> QVQSVEVMRDSYGVPHVFADSHYGLYYGYGYAVAQDRLFQMDMARRSFVGTTAAVLGPGEQDAYVKYDMQVRQNFTPASIQRQIAALSKDERDIFRGYADGYNAYLEQVRRRPELLPKEYVDFDFQPEPLTDFDVVMIWVGSMANRFSDTNLEVTALAMRQSLEKQHGPERGRALFDELLWINDTTAPTTVP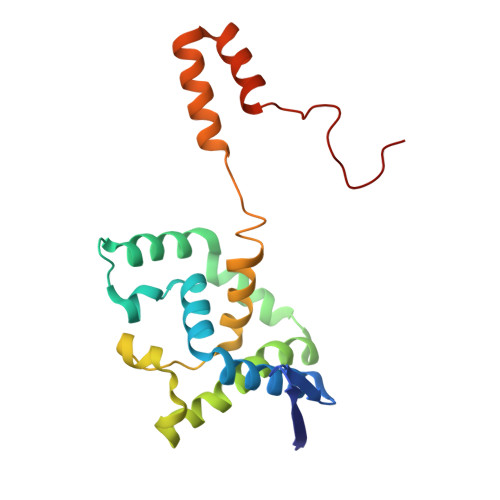APA> MGSSHHHHHHSQDPMLNSFKLSLQYILPKLWLT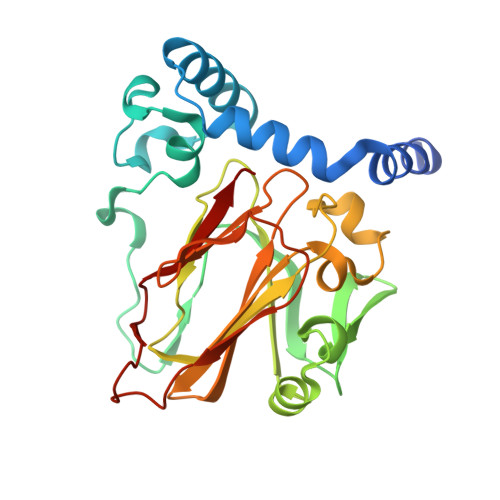RLAGWGASKRAGWLTKLVIDLFVKYYKVDMKEAQKPDTASYRTFNEFFVRPLRDEVRPIDTDPNVLVMPADGVISQLGKIEEDKILQAKGHNYSLEALLAGNYLMADLFRNGTFVTTYLSPRDYHRVHMPCNGILREMIYVPGDLFSVNHLTAQNVPNLFARNERVICLFDTEFGPMAQILVGATIVGSIETVWAGTITPPREGIIKRWTWPAGENDGSVALLKGQEMGRFKLG> MGLVENIKQFNDAVSSVKPGDEIVLANGSWNDVELVLKGKGLPDKPITLKAQTPGKVIITGQSNLAFSGEYIVISGLVFKDGATPTGEVISFRTSNEDVANHSRVTNTVIDNFSTDLRQMSDLWVAMYGKHNRLDHNSLVNKRNRGVTVAVRMNSEASRKNHHIIEYNYFGPRQILGANGGETLRIGTSHFSREYSNTTAQYNYFDRTNGEHEIISNKSSGNSLIKNVFFETQGTLTMRHGHFTKVEGNYFLGNRKPNTGGIRIINESQTVSNNYMYGLTGKRLRGALVIMNGVPNSPPNRYDPVIDSAMNNNIVIDSDHIELGAGADAERSAAPSTSEFKGNIILGKSNLEPFTLYDDMSGINFEGNYLNDEASTPIKTGFASTPYSVTTNQYGLKSPDKALLDEIGFGEVKLPVTKEEVGADFYPKNEALVAFQSGKTIHVKAGTDTLTSALATSQGGDVLVLENGADYLLTKFAEVHHPVTIMAKAGKKPVIRSQKPNFINIENGGA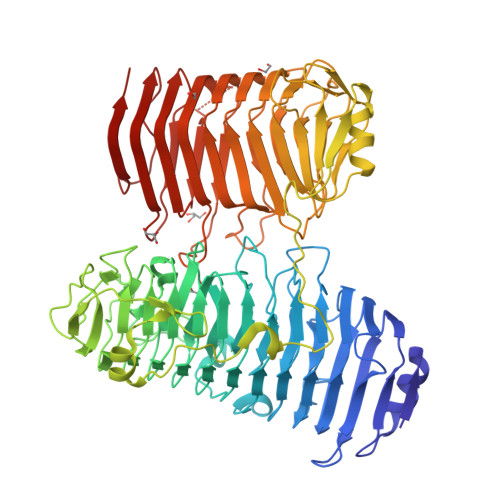LEVENLWFDGAESPDYKGNTIIGTSGYSMNINYNLSVRNVKVTDLDVNGYFYFFKANAGTFADSIEIIDSEFSNITGAILQLNREVDDLGVYSVENLVISGNTFTNVKEEVVTVYRGGTDESTFGPMVSVTNNTLTNVGKGSTHRSGASMYFHGVQKLNISETKWDNSAPLELFLTNGGPITVIDNVEMKNTDKIRANNDEYESSNVTYD>GPGSMTDFYSLIPSAPKGRFDGIERAHTAEDVKRLRGSVEIKYSLAEMGANRLWKLIHEEDFVNALGALSGNQAMQMVRAGLKAIYLSGWQVAADANTASAMYPDQSLYPANAGPELAKRINRTLQRADQIETAEGKGLSVDTWFAPIVADAEAGFGGPLDAFEIMKAYIEAGAAGVHFEDQLASEKKCGHLGGKVLIPTAAHIRNLNAARLAADVMGTPTLIVARTDAEAAKLLTSDIDERDQPFVDYEAGRTAEGFYQVKNGIEPCIARAIAYAPYCDLIWMETSKPDLAQARRFAEAVHKAHPGKLLAYNCSPSFNWKKNLDDATIAKFQRELGAMGYKFQFITLAGFHQLNYGMFELARG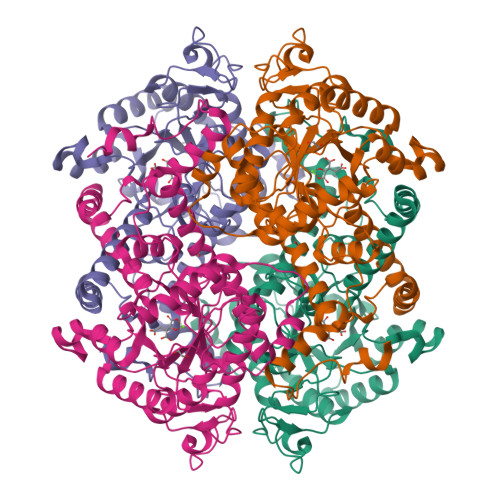YKDRQMAAYSELQQAEFAAEADGYTATKHQREVGTGYFDAVSLAITGGQSSTTAMKESTETAQFKPAAE[4x]>[2x]GSHMSVRIVDVREITKPISSPIRNAYIDFTKMTTSLVAVVTDVVREGKRVVGYGFNSNGRYGQGGLIRERFASRILEADPKKLLNEAGDNLDPDKVWAAMMINEKPGGHGERSVAVGTIDMAVWDAVA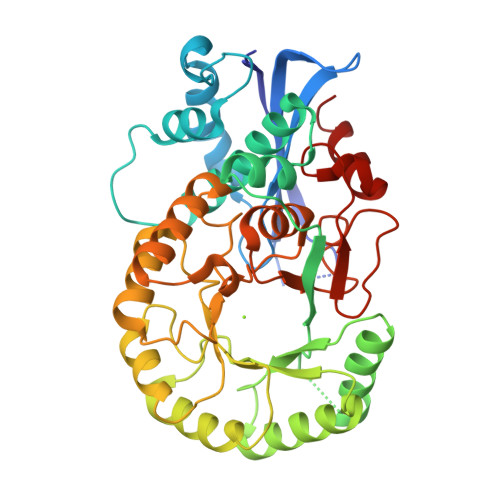KIAGKPLFRLLAERHGVKANPRVFVYAAGGYYYPGKGLSMLRGEMRGYLDRGYNVVKMKIGGAPIEEDRMRIEAVLEEIGKDAQLAVDANGRFNLETGIAYAKMLRDYPLFWYEEVGDPLDYALQAALAEFYPGPMATGENLFSHQDARNLLRYGGMRPDRDWLQFDCALSYGLCEYQRTLEVLKTHGWSPSRCIPHGGHQMSLNIAAGLGLGGNESYPDLFQPYGGFPDGVRVENGHITMPDLPGIGFEGKSDLYKEMKALAE(2R,3R,4S)-2-(hydroxymethyl)-1-[(4-hydroxythieno[3,2-d]pyrimidin-7-yl)methyl]pyrrolidine-3,4-diol | C12 H15 N3 O4 S | 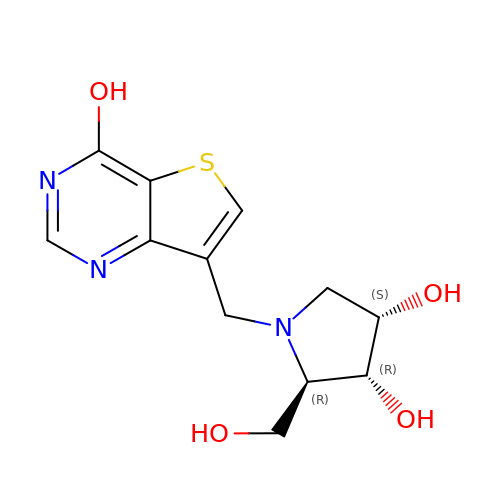UZJHCHSHAYEOTK-KHQFGBGNSA-N Human T-cell Leukaemia Virus type 1 (HTLV-1) is an untreatable retrovirus that causes lethal malignancies and degenerative inflammatory conditions. Here, we show that high-resolution crystal structures of the mature-length HTLV-1c CA protein define essential lattice interfaces and identify a distinct ligand-binding pocket. Across the known Orthoretrovirinae, CA is a two-domain protein with HIV being the best characterised. However, our structures reveal that HTLV-1 does still have a pocket formed between helices 3, 4, and 5, albeit an electropositive one capable of binding to either phosphate or sulfate in vitro.

The full-length HTLV-1 CA protein was solved to a resolution of 2.25 Å in space group F222 with three molecules in the asymmetric unit. Applying a crystallographic 2-fold rotation generated the CA hexamer, packed as sheets, effectively identical to those observed in the hexagonal crystal form of the CANTD (RMSD = 1.143 Å). Despite the high resolution, the electron density for the CTD was of lower quality with a higher B-factor compared with the NTD, suggesting that it remains flexible relative to the NTD in the crystal. To improve the CA full-length structure, we re-solved it by molecular replacement searching for three independent copies of the refined CACTD structure as a search model. This unbiased approach returned a CTD dimer virtually identical to that mediated by α-helix 9 in the CACTD structure (RMSD = 1.580 Å), suggesting that this is the biologically relevant dimer interface. In the HTLV lattice, the NTD mediates both intra- and inter-hexamer interactions. The CTD is excluded from the NTD plane, but also contributes inter-hexamer interactions through CTD dimerization. This results in a closer-packed lattice for HTLV, with a distance between hexamer centres of 74.6 Å, nearly 20 Å shorter than that of the HIV lattice (92.0 Å). While there is currently no equivalent structure available for the HTLV-1 mature CA lattice, the comparison strongly suggests that our HTLV-1c CA crystal structure packing most closely resembles the immature lattice. As such, it is plausible that the full-length HTLV-1c CA crystal structure represents a maturation intermediate.

>PVMHPHGVPPSHRPWQMKDLQAIKQEVSQAAPGSPQFMQTIRLAVQQFDPTAKDLQDLLQYLCSSLVASLHHQQLDSLISEAETRGITGYNPLAGPLRVQANNPQQQGLRREYQQLWLTAFAALPGSAKDPSWASILQGLEEPYHTFVERLNVALDNGLPEGTPKDPILRSLAYSNANKECQKLLQARGHTNSPLGDMLRACQAWTPKDKTKVL[3x]> ADDEKNALPISKDGYIRVPKERVNVNLTSIKKLREKVDDSIHRELTDIFANLNYVGVVDEERRLAAIQHDLKLFLIDYGSVCYELFYQIGLTDFANFGKINLQSTNVSDDIVLYNLLSEFDELNDDASKEKIISKIWDMSSMLNEYYSIELVNDGLDNDLKSVKLKSLPLLLKGYIPSLVKLPFFIYRLGKEVDWEDEQECLDGILREIALLYIPDMVPKVDTSDASLSEDEKAQFINRKEHISSLLEHVLFPCIKRRFLAPRHILK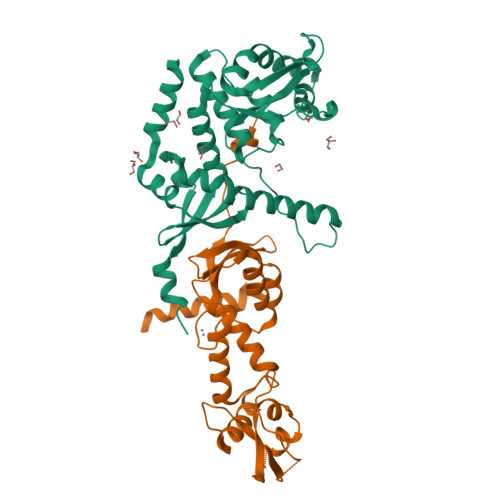DVVEIANLPDLYKVFERC;> SKRKSEAQENIIKNKDELEDFEQGEKYLTLTVSKNDFKKMEVVGQFNLGFIIVTRKVDNKYDLFIVDQHASDEKYNFETLQAVTVFKSQKLIIPQPVELSVIDELVVLDNLPVFEKNGFKLKIDEEEEFGSRVKLLSLPTSKQTLFDLGDFNELIHLIKEDGGLRRDNIRCSKIRSMFAMRACRSSIMIGKPLNKKTMTRVVHNLSELDKPWNCPHGRPTMRHLMELRDWSSFSKDYEI> MGSSHHHHHHSQAPIEGRAQVINTFDGVADYLQTYHKLPDNYITKSE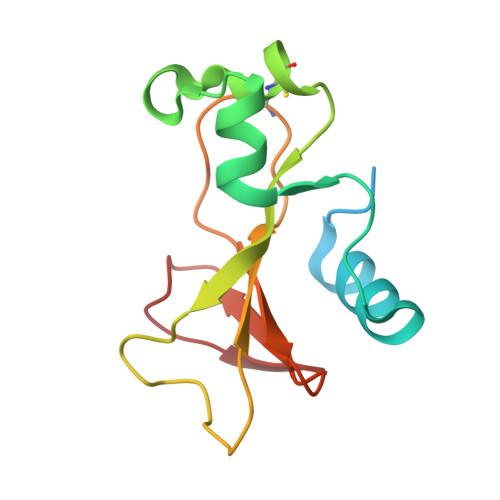AQALGWVASKGNLCDVAPGKSIGGDIFSNREGKLPGKSGRTWREADINYTCGFRNSDRILYSSDWLIYKTTDHYQTFTKIR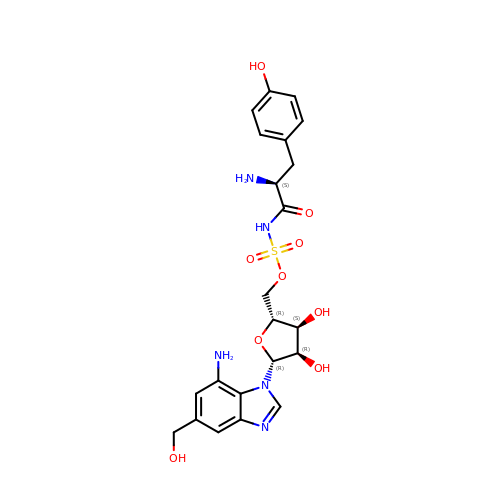[(2~{R},3~{S},4~{R},5~{R})-5-[7-azanyl-5-(hydroxymethyl)benzimidazol-1-yl]-3,4-bis(oxidanyl)oxolan-2-yl]methyl ~{N}-[(2~{S})-2-azanyl-3-(4-hydroxyphenyl)propanoyl]sulfamate | C22 H27 N5 O9 S | BKJCUHPLMCZZDC-JZACSSPNSA-N>[5x]GQDMVSPPPPIADEPLTVNTGIYLIESYSLDDKAETFKVNAFLSLSWKDRRLAFDPVRSGVRVKTYEPEAIWIPEIRFVNVENARDADVVDISVSPDGTVQYLERFSARVLSPLDFRRYPFDSQTLQIYLIVRSVDTRNIVLAVDLEKVGKNDDVFLTGWDIESFTAVVKPANFALEDRLESKLDYQLRISRQYFSYIPNIILPMLFILFISWTAFWSTSYEAN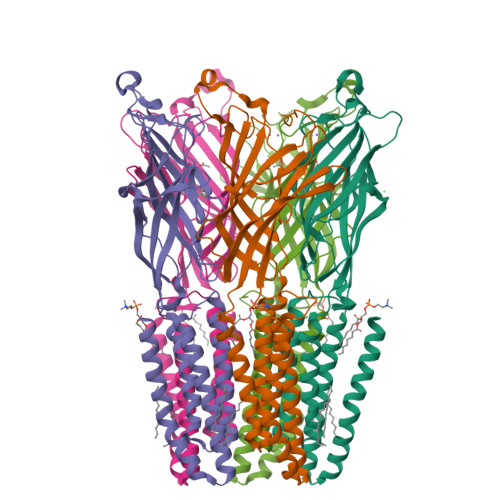VTLVVSTLIAHIAFNILVETNLPKTPYMTYTGAIIFMIYLFYFVAVIEVTVQHYLKVESQPARAASITRASRIAFPVVFLLANIILAFLFFGF> GSMSESADLTELYSIIEKTAQVVDVTASHDKVWPILNAFQDVIADSVISFRASTGSSADDLDCRFTMLPKGLDPYARALEHGLTPKTDHPVGSLLKEVHENLPITSCGVDFGVAGGFTKTWSFPSAEKLGKVSELVKLPSIPDAVAANRDFFEKWGIADMVSTVGID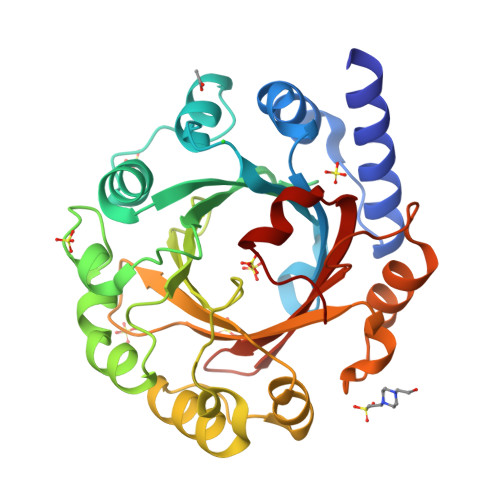YSKRTMNLYFGGGVGDRVPAGVFEEKGVRAILGELGLAAPSEELLKFCERSFVIYVTLSWDSPKINRFTYSVMTPEPLGLPVDLAPTFERLIKSAPYDTEGRNYVYGIASTPKGEYHKIASYYQWQKRVEKLLRSDG>[3x]MEMLTKFESRSSRAAGVAFHPTQPWILTSLHNGRIQLWDYRMGTLLDRFDGHDGPVRGIAFHPTQPLFVSGGDDYKVNVWNYKSRKLLFSLCGHMDYVRVCTFHHEYPWILSCSDDQTIRIWNWQSRNCIAILTGHSHYVMCAAFHPSEDLIVSASLDQTVRVWDISGLRMKNAAPVSMSKEDQKAQAHNSKSNDKKGSTDAIVKFVLEGHDRGVNWCAFHPTLPLILSAGDDRLVKLWRMTASKAWEVDTCRGHFNNVSCCLFHPHQELILSASEDKTIRVWDLNRRTAVQTFRRDNDRFWFITVHPKLNLFAAAHDSGVMVFKLESAWSHPQFEK

Hence, this loss of critical proteins has the potential to compromise ER proteostasis and generate cellular stress. This challenge to normal metabolism is overcome by the activity of the cytosolic coatomer protein I (COPI) polymer, whose repeating unit is the coatomer, a 560 kDa complex of seven distinct gene products (α-, β-, β′-, γ-, δ-, ε-, and ζ-COPI)25–31. Overall, the coatomer functions to retrieve the escaped “client” proteins, such as type I membrane proteins, from cis-Golgi back to ER by retrograde trafficking. In particular, the S protein – a type I membrane protein – is delivered to the ERGIC from both the ER (by anterograde trafficking) and the Golgi (by retrograde trafficking)3,10–12. Here we utilize recombinant SARS-CoV-2 S proteins and tail peptides, including constructs with enhanced mimicry of the coatomer binding motif (clientized S protein), to elucidate the atomic structure of the S-coatomer interface.

To gain insight into the role of the basic cluster in stabilizing S-coatomer interactions, we generated alanine mutants of αWD40 Arg13, Lys15, and Arg300, which are equivalent to the β‘WD40 basic cluster residues Arg15, Lys17, and Arg272, respectively. Finally, the Lys15Ala mutant did not bind to either the wild-type or clientized Thr1273Glu S heptapeptides, and a 1.6 Å resolution crystal structure revealed this was due to conformational occlusion of the αWD40 binding site by an inward rotation of nearby Arg13 and His31 side chains, rather than loss of Lys15 interactions. L Superposition of wild-type (white) and Lys15Ala mutant (yellow) crystal structures shows substantial perturbation and inward rotation of Arg13 and His31 side chains in the mutant to block the S heptapeptide binding site. We therefore generated wild-type and clientized Thr1273Glu S heptapeptides with amidation at the C-terminal main chain carboxylate, which neutralizes the main chain charge that interacts with αWD40 Lys15. This approach does not perturb the binding site architecture of αWD40, unlike mutagenesis. Loss of αWD40 binding was observed for the amidated wild-type S heptapeptide but not the amidated clientized Thr1273Glu S heptapeptide. In contrast, Arg13 and Lys15 residues in αWD40 provide the basis for basal binding to both wild-type and clientized S molecules.~{N}-[2-[5-chloranyl-2-[(1-methylpyrazol-4-yl)amino]pyrimidin-4-yl]oxyphenyl]prop-2-enamide 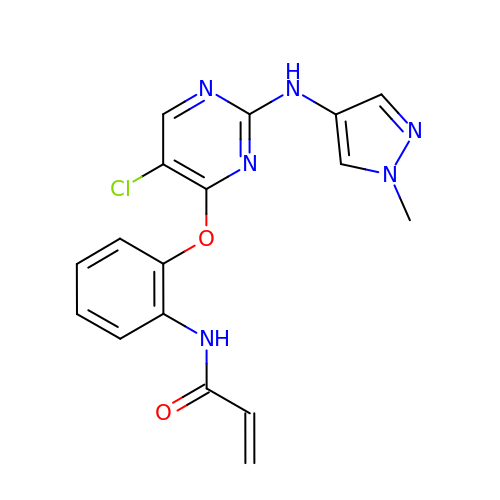| C17 H15 Cl N6 O2 | QXQGHCJUTRTRLJ-UHFFFAOYSA-N>MNVLSVSSEIYPLIKTGGLADVVGALPIALEAHGVRTRTLIPGYPAVKAAVTDPVKCFEFTDLLGEKADLLEVQHERLDLLILDAPAYYERSGGPYLGQTGKDYPDNWKRFAALSLAAARIGAGVLPGWRPDMVHAHDWQAAMTPVYMRYAETPEIPSLLTIHNIAFQGQFGANIFSKLALPAHAFGMEGIEYYNDVSFLKGGLQTATALSTVSPSYAEEILTAEFGMGLEGVIGSRAHVLHGIVNGIDADVWNPATDHLIHDNYSAANLKNRALNKKAVAEHFRIDDDGSPLFCVISRLTWQKGIDLMAEAVDEIVSLGGRLVVLGAGDVALEGALLAAASRHHGRVGVAI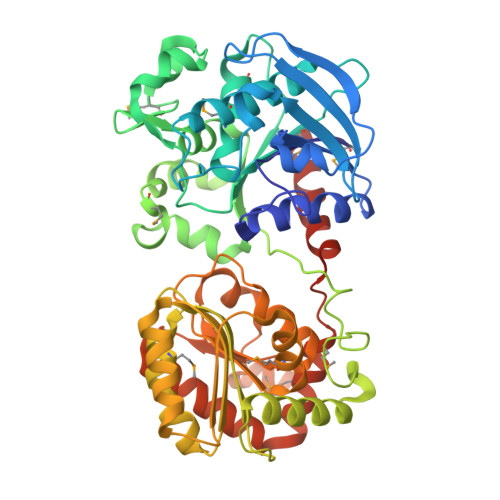GYNEPLSHLMQAGCDAIIIPSRFEPCGLTQLYALRYGCIPVVARTGGLADTVIDANHAALASKAATGVQFSPVTLDGLKQAIRRTVRYYHDPKLWTQMQKLGMKSDVSWEKSAGLYAALYSQLISKGHHHHHH[2x]>[2x]MKTFAAYVIIACLSSTALA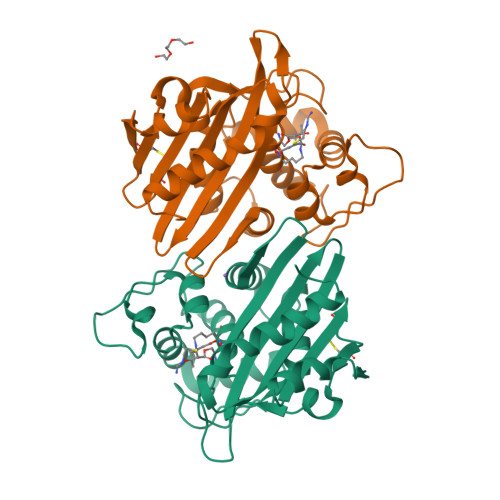GSITENTSWNKEFSAEAVNGVFVLCKSSSKSCATNDLARASKEYLPASTFKIPNAIIGLETGVIKNEHQVFKWDGKPRAMKQWERDLTLRGAIQVSAVPVFQQIAREVGEVRMQKYLKKFSYGNQNISGGIDKFWLEGQLRISAVNQVEFLESLYLNKLSASKENQLIVKEALVTEAAPEYLVHSKTGFSGVGTESNPGVAWWVGWVEKETEVYFFAFNMDIDNESKLPLRKSIPTKIMESEGIIGG> MAGLPRRIIKETQRLLAEPVPGIKAEPDESNARYFHVVIAGPQDSPFEGGTFKLELFLPEEYPMAAPKVRFMTKIYHPNVDKLGRICLDILKDKWSPALQIRTVLLSIQALLSAPNPDDPLANDVAEQWKTNEAQAIETARAWTRLYAMNNI;> SHSGFKCPICSKSVASDEMEMHFIMCLSKPRLSYNDDVLTKDAGECVICLEELLQGDTIARLPCLCIYHKSCIDSWFEVNRSCPEHPAD

E3 ligases catalyze the final step in this cascade by promoting the transfer of activated Ubs from E2∼Ub thioester intermediates to specific substrates or to the growing ends of substrate-linked Ub chains. One such study carried out by Hoxhaj et al. found that RING E3 ligase ZNRF1 co-purifies with Ube2N from transiently transfected HEK293 cells in stoichiometric amounts. This E3 ligase was first identified as one of the gene products up-regulated in Schwann cells upon peripheral nerve injury and contains a Zinc-finger (ZnF) domain juxtaposed to its C-terminal RING domain. Though the precise cellular roles of ZNRF1 remain to be deciphered, it has been found to co-localize with tubulin in cells and ubiquitinates protein kinase B (Akt1), glutamine synthase, and the α subunit of Na+/K+ pump. Our results reveal that despite having a canonical E3 : E2 interaction, mediated exclusively by the RING domain, ZNRF1/Ube2N interface is ‘tuned’ at the molecular level to achieve unprecedented nanomolar affinity.

Accordingly, we prepared the C-terminal domain of ZNRF1, ZNRF1CTD, comprising residues 139–227 of the full-length protein. Experiments reveal that Ube2N binds ZNRF1CTD with a dissociation constant (Kd) of ∼39 nM at 25°C. Crystals were successfully obtained in the P212121 space group and allowed us to collect a 1.47 Å dataset. The structure solved using the anomalous signal from the Zn2+ atoms contains one molecule of ZNRF1CTD in the asymmetric unit of the crystal together with one molecule of Ube2N bound to the RING domain in a canonical manner. The ∼520 Å2 interface area of the ZNRF1 : E2 interface is also comparable to most RING E3 : E2 complexes solved till date. ZnF domain contributes minimally in engaging Ube2N in the canonical manner, but contacts a symmetry-related Ube2N molecule in the crystal facilitating crystal packing. Moreover, binding of ZnF to Ube2N as observed in our crystal occludes the activated Ub to adopt closed conformation required for the catalysis. The analysis reveals that ZNRF1 : Ube2N interface contains three salt-bridges/H-bonds involving Glu183 of ZNRF1 and Arg14/Lys10 of Ube2N. Besides these residues, our complex structure solved just shy of 1.5 Å, underscores the importance of several other H-bonding/salt-bridges between various side-chains and main-chain peptide moieties, water-mediated H-bonding interactions, and hydrophobic residues such as Met64 in E3 : E2 interactions dictating the overall affinity. In addition, the water-mediated H-bonding was particularly intriguing in our case as no such water-mediated bonds have been observed in any of the E3–E2 crystal structures.>LHNYGYTSTKSVDNQIEELREKVVSKNKNEPEFLQAFEEVLSCLKPVFKKDNVYIGVLENIAEPERVIQFRVPWINDKGEHKMNRGFRVQYNSVLGPYKGGLRFHPAVNLSVIKFLGFEQIFKNSLTTLPMGGGKGGSDFDPKGKSENEILKFCQSFMTNLFRYIGPNTDVPAGDIGVGGREIGYLFGQYKKLKNSFEGVLTGKNIKWGGSNIRAEATGYGVVYFAENVLKDLNDNLENKKCLVSGSGNVAQYLVEKLIEKGAIVLTMSDSNGYILEPNGFTKEQLNYIMDIKNNQRLRLKEYLKYSKTAKYFENQKPWNIPCDIAFPCATQNEINENDADLFIQNKCKMIVEGANMPTHIKALHKLKQNNIILCPSKAANAGGVAVSGLEMSQNSMRLQWTHQETDMKLQNIMKSIYEQCHNTSKIYLNESDLVAGANIAGFLKVADSFLEQ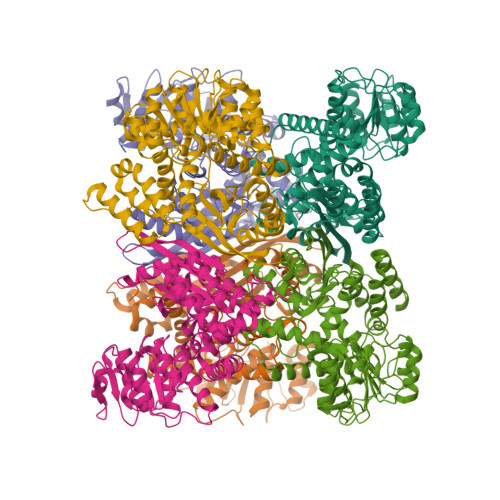GGL[6x]> TDYTKYVNTFIGAADNGHTFPGACRPFGMIQTSPVTGAVGWRYCSEYVNSDSIIWGFTQTHLNGTGCMDLGDVLVMPVTGTRTRAWDAYRSRFSKKLEAATPGYYTVELTEPNVKAELTATPHAALHRYTYHNADSASVLIDLQHGPTWNENQYHSQVKECEVNWEDAQTLTGHVRNSVWVNQDYFFVMKFNRPVTDSLYLPMGETEKGKRIIASFDMQPGEELLMKVALSTTGIEGARKNMEAEVPAWDFEGVKKTAHDDWNSYLSRIDVTGTEDEKTNFYTCFYHALIQPNQISDVDGLYRNAADSVVKAGTGTFYSTFSLWDTYRAAHPFYTLMVPEKVDGFVNSLVEQSEVQGFLPIWGLWGKETYTMVGNHGVSVIAEAYRKGFRGFDAERAFNAIKQT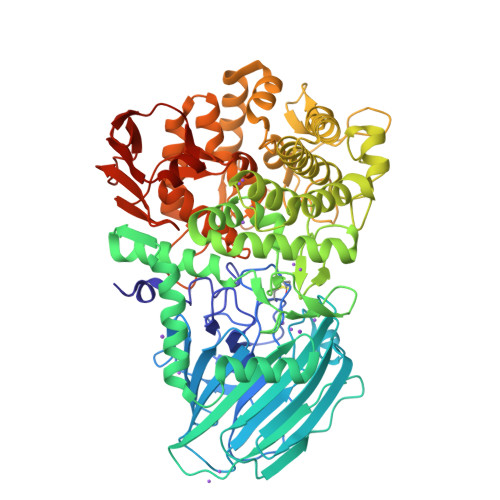QTVSHKQKSDWETYMKYGYFPTDLIKTESVSSSLESVYDDYAAADMAKRMGKTEDAAYFSKRADFYKNLFDTETQFMRPRNSNGTWKTPFNPSQVAHAESTGGDYTEGNAWQYTWHVQHDVPGLISLFGGEEPFLNKLDSLFTLKLETTQADVTGLIGQYAHGNEPSHHITYLYALAGRPERTQELVREIFDTQYHPEPDGLCGNDDCGQMSAWYMFSAMGFYPVDPVSGNYVFGAPQMPKIVLHLADGKTFTVIADGISKEHKYIDSITLNGEPYTKNYISHEDILKGGTLVYKMKLEHHHHHH>MATSASSHLNKGIKQVYMSLPQGEKVQAMYIWIDGTGEGLRCKTRTLDSEPKGVEELPEWNFDGSSTFQSEGSNSDMYLVPAAMFRDPFRKDPNKLVFCEVFKYNRKPAETNLRHTCKRIMDMVSNQHPWFGMEQEYTLMGTDGHPFGWPSNGFPGPQGPYYCGVGADKAYGRDIVEAHYRACLYAGIKIAGTNAEVMPAQWEFQIGPCEGIDMGDHLWVARFILHRVCEDFGVIATFDPKPIPGNWNGAGCHTNFSTKAMREENGLKYIEESIEKLSKRHQYHIRAYDPKGGLDNARRLTGFHETSNINDFSAGVANRGASIRIPRTVGQEKKGYFEDRRPSANCDPF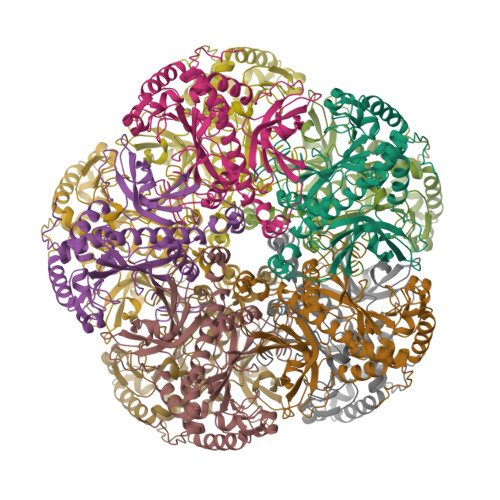SVTEALIRTCLLNETGDEPFQYKNLEHHHHHH[15x]>RSWHYVEPKFLNKAFEVALKVQIIAGFDRGLVKWLRVHGRTLSTVQKKALYFVNRRYMQTHWANYMLWINKKIDALGRTPVVGDYTRLGAEIGRRIDMAYFYDFLKDKNMIPKYLPYMEEINRMRPADVPVKYMGK[4x];>AQTNAAADWDVYCSQDESI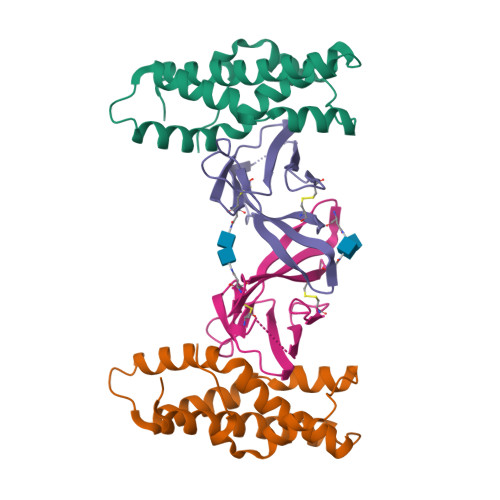PAKFISRLVTSKDQALEKTEINCSNGLVPITQEFGINMMLIQYTRNELLDSPGMCVFWGPYSVPKNDTVVLYTVTARLKWSEGPPTNLSIQCYMPKSPVAPKLEHHHHHH[4x]> AAAAAAAAAAAAAAAAAA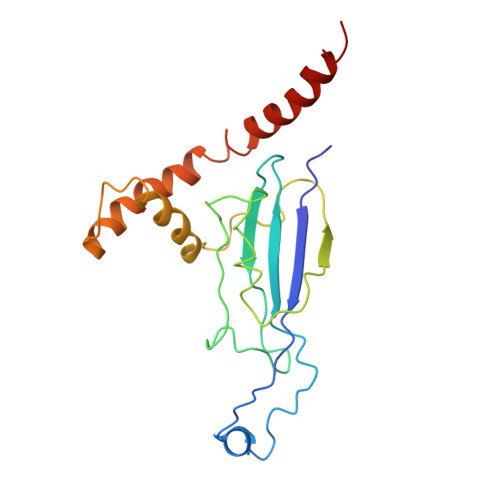AAAAAAAAAAAAAAAAAAAAAAAAAAAAAAAAAAAAAAAAAAAAAAAAAAAAAAAAAAAAAAAAAAAAAAAAAAAAAAAAAAAAAAAAAAAAAAAAAAAAAAAAAAAAAAAAAAAAAAAAAAAAAAAAAAAAAAAAAAAAAAAAAAAAAAAAAAAAAAAAAAAAAAAAA>[2x]MQKTF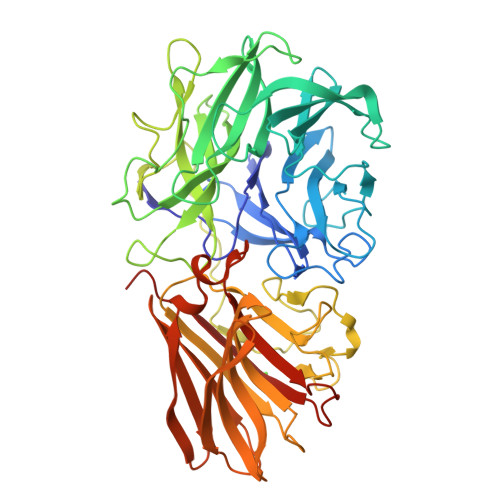RNPIITGMNPDPSICRVGDDFYLVTSTFEYFPGLPVYHSKDLVHWKLIGHALSRPENNPLMGCNASTGGQYAPTLRYHDGTFYVIGTNYGGKGSQGVFYVTAKNPAGPWSDPVWVGNWYVDPSIEFIDGKMYFLSPDNQGSFLLGVMDPETGTFVEALRKVASGLGGSSPEGPHFYKIGDYYYIMSAEGGTGYEHREVIQRSKSPWGPYEPSPVNPVLSNMNCPDHPFQAIGHADLVQLKDGSWWAVCLGIRPVNGKYQHLGRETFLAPVTWDADGWPKVGKDGVVQETYLFPNLPSHVWMEQPVRDDFDQETLGLDWTFIRNPAHSFWSLTEKPGSLRLKGTAINFTTNDSPSFIGRRQAAFNLTASAKVNFIPKVENEEAGLVVRADDKNHYDLLITERNGQRVAMIRKTLKDKVVDTTCKELPATGEVILSITATETTYTFEIKAAHVSAILGTASTRDVSNEVVGGFTGVFIGMYASGNGQANTNPADFDWFDFRCLDLEHHHHHH In particular, the superlectin BC2L-C is believed to cross-link human epithelial cells to B. cenocepacia during pulmonary infections. BC2L-C was also found to contain an N-terminal trimeric domain, which features specific millimolar affinity for L-fucose and high micromolar affinity for fucosylated histo-blood oligosaccharides. Thus, BC2L-C presents a double carbohydrate specificity, maintained through a hexameric assembly, which makes it a superlectin, hypothesized to crosslink cells by simultaneously binding bacterial mannosides in its C-terminal domain and human fucosides in the N-terminal domain. The first generation of antagonists was thus designed as a panel of β-C- and β-N-fucoside glycomimetic bifunctional molecules, simultaneously targeting BC2L-C-Nt’s carbohydrate binding site and its neighboring site.

We solved two new crystal structures featuring complexes of BC2L-C-Nt with synthetic ligands 22a and 8c, allowing further rationalization of the affinity observed. The structures resulted from soaking BC2L-C-Nt crystals for 24 h in a 1.25 mM solution of each ligand and were solved to 1.79 and 1.32 Å resolution by molecular replacement. In the structure featuring ligand 22a, the alkyne linker is 4.1 Å long and does not significantly dislocate the nearby crystallographic water W2 (top). The fragment’s aromatic moiety engages in the predicted π/π T-shaped interaction with Tyr58, with an edge-to-face distance of 3.9 Å between its centroid and the closest C-atom of Tyr58 side chain, albeit the angle is 58°, rather than 90° (top). Instead of the salt bridge predicted by docking, a water-mediated contact between Asp70 and the amino group is observed (top). Other characteristics of this interaction include the shape complementarity of hydrophobic patches: both methyl groups of the fragment are in close proximity with the otherwise exposed hydrophobic surface generated by the main chain of Gly71 and side chain of Tyr58. This hydrophobic complementarity carries on to match with residues Cys72, Thr46, and Ser119. Alternatively, 22a with a KD of 281 μM was identified as the main hit with suitable values in both SPR and ITC and a nearly 10-fold affinity increase from αMeFuc. Additionally, we can rationalize the affinity gain observed for hit structure 22a as the result of three factors: (1) the T-shaped π/π interaction, (2) the shape complementarity between hydrophobic surfaces, and (3) the thermodynamically advantageous entropic factor.

> GHMPLLSASIVSAPVVTSETYVDIPGLYLDVAKAGIRDGKLQVILNVPTPYATGNNFPGIYFAIATNQGVVADGCFTYSSKVPESTGRMPFTLVATIDVGSGVTFVKGQWKSVRGSAMHIDSYASLSAIWGTAA trans-3-({4-(cyclohexylmethyl)-5-[3-(1-methylcyclopropyl)-5-{[(2R)-1,1,1-trifluoropropan-2-yl]carbamoyl}phenyl]-1,3-thiazole-2-carbonyl}amino)cyclobutane-1-carboxylic 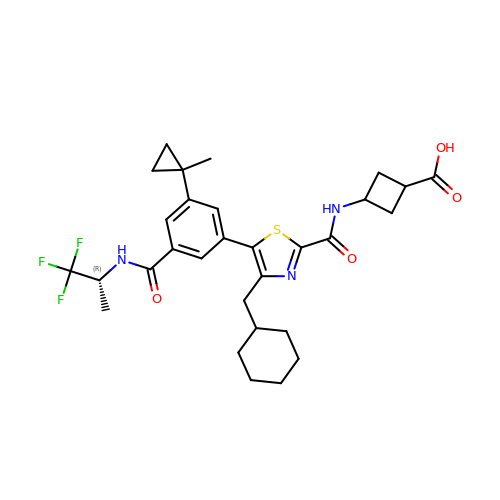acid | C30 H36 F3 N3 O4 S | PSFPATVFAWGHAJ-BSLALVQMSA-N>[2x]GIDPFTDDLEQYLDEKILRLKDEMNIAAQLDIDTLNKRIETGDTSLIAMQKVKLLPKVVSVLSKANLADTILDNNLLQSV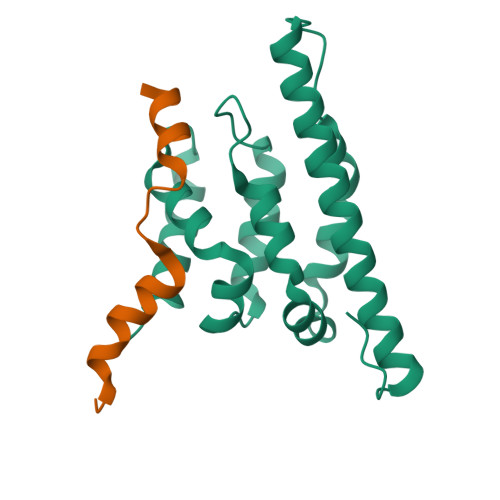RIWLEPLPDGSLPSFEIQKSLFAALNDLPVKTEHLKESGLGRVVIFYTKSKRVEAQLARLAEKLIAEWTRP;>DPFTHMSDKIDEMYDIFGDGHDYDWALEIEN[2x]> LPGEGTQVHP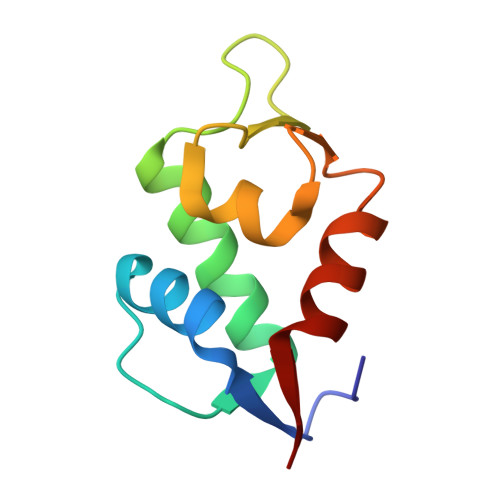RAPLLQILKVAGAQEEVFTVKEVMHYLGQYIMMKQLYDKQRQHIVHCHDDPLGELLEVGSFSVKNPSPLYEMLKRNLVIL> MATRLDRLVTILETGSTRLIRDTAVNQLADWQKQHPEELFNLLSRVVPYLRHKDWETRTTAAKAIGKIIENAPLYDPNAGQDEAAPEPTNGSFEVKKEEEKDVLEQDNFFRLESLDVATIVKYGRPLLRGGPVDYNLAALDPQKRLAHLKKTLNGRLGLLGRVFEDEEMPVEQIASPITPNDAAGANGVGRQDGASNDNQSQAIDESKMSARQLNVLKRKRKREAQKAAQGKSGFGDLSLRRSTTAGSDAFGEDTPMPDADSKKNKLAEYFSLDRPENTEEDTKIVSEFKGPVLPIKSEIEADDSLEGAEWPFERLCEFLKVDLFDPQWETRHGAAMGLREVIRVHGAGAGRRRGKTRKENNDLNRQWLDDLAYRLLCVLMLDKFTDYSSDTSVAPIRETVGQTLGAVLRHISVESVHAIYRLLYCMVTQEDLPSEQNMWAVCHGGMVGLRYVVAVRKDLLLQDGDMIDGVVRCVMQGLGDIDDDVRSVSAATLIPMAKEFVMMRRSALDSLINIVWESLSNLGDDLSASTGKIMDLLATLCSFPEVLEAMKVSASQDEERSFTLLVPRLYPFLRHTITSVRLAVLKALMTFANLGGETSQGWLNGRILRLIFQNIIVERDQDTLNMSLELWTTLVRRLAARDPAILADEFEAHAEPMMQLALHPIGVPRHPIPMNPALFQKPSGGTYSLPGASQTNSRRSSPPEGERATKRRRKSTKAEDVAPSTHTHDVDGHMIQGEVDLVGVDVLIRSRISAAKAMGLIMSFIPTPRLASYDTAVLQALSSPYASTQLAAAMVIDEYAKNCSTPEVASRFIEPLQKIIDLERPSHYRDLVTYVQRVRSASQQLINLFRDHGKVSQGKLPTLAVVVQGEPEAGPGAFSIANAEKVVNEDFERLKRLMAPGQRLIALPQLNEAREQTVEVIEEAKAAKEARDARIKAAAACALVAMKVLPKKPSPLIKAIMDSIKTEENQELQSRSAATIARLVQLFTESGRRGPAEKVVANLVKFSCVEVAETPEFPIHAHKTNVILSMQKEEDRVDHPDAVKYAREAKAARITRRGAKEALEILSKNFGAELLERVPTLRTFMEEPLVRAFSGDLPPEARDPENAFGQEIVDAMSVIRTMTPTLHPALHPFVMQQVPLVIKALRSDLSVFRYMAAKCMATICSVITVDGMTALVEKVLPSINNPLDLSFRQGAIEVIYHLIAVMGDAILPYVIFLIVPVLGRMSDSDNQIRLIATTSFATLVKLVPLEAGIPDPPGLSEELLKGRDRERTFIAQLLDPKKIEPFKIPVAIKAELRSYQQEGVNWLAFLNKYHLHGILCDDMGLGKTLQTICIVASDHHQRAEEFARTGAPEVRKLPSLIICPPTLSGHWQQEIKTYAPFLTVTAYVGSPAERRAMKDSLDKTDIVITSYDVCRNDIDVIEKYNWNYCVLDEGHLIKNPKAKITLAVKRLTSNHRLILTGTPIQNNVLELWSLFDFLMPGFLGAEKVFLDRFAKPIANSRYSKASSKEQEAGALAIEALHKQVLPFLLRRLKEEVLNDLPPKILQNYYCDLSDLQRKLFEDFTKREGKKITETAGRDDKEAKQHIFQALQYMRKLCNSPALVMKPGHKAYEDTQKYLAKHGTTLEDPIHAPKLGALRDLLVDCGIGVEGQESSDPLYTPIKPHRALIFCQMKEMLDMVQNTVLKQMLPSVSYLRLDGSVEANKRQDIVNKFNSDPSYDVLLLTTSVGGLGLNLTGADTVIFVEHDWNPQKDLQAMDRAHRIGQKKVVNVYRIITRGTLEEKILSLQRFKIDVASTVVNQQNAGLATMDTDQILDLFNLGESGPSLITDNKE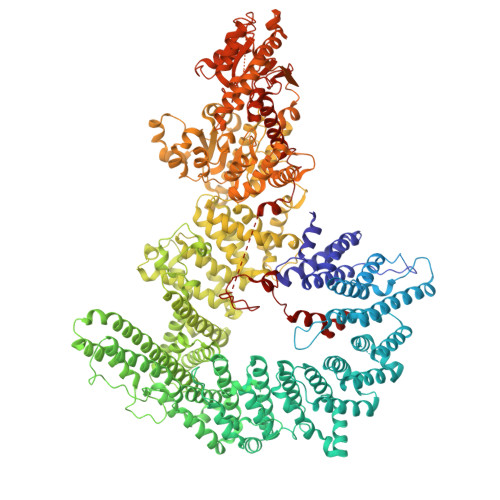SIEGREEDMVDIETGDVRRPGKKAAWLEGLGELWDNAQYEESFDLDGFLKTMQAAAWSHPQFEK> MAMITGGELVVRTLIKAGVEHLFGLHGAHIDTIFQACLDHDVPIIDTRHEAAAGHAAEGYARAGAKLGVALVTAGGGFTNAVTPIANAWLDRTPVLFLTGSGALRDDETNTLQAGIDQVAMAAPITKWAHRVMATEHIPRLVMQAIRAALSAPRGPVLLDLPWDILMNQIDEDSVIIPDLVLSAHGARPDPADLDQALALLRKAERPVIVLGSEASRTARKTALSAFVAATGVPVFADYEGLSMLSGLPDAMRGGLVQNLYSFAKADAAPDLVLMLGARFGLNTGHGSGQLIPHSAQVIQVDPDACELGRLQGIALGIVADVGGTIEALAQATAQDAAWPDRGDWCAKVTDLAQERYASIAAKSSSEHALHPFHASQVIAKHVDAGVTVVAD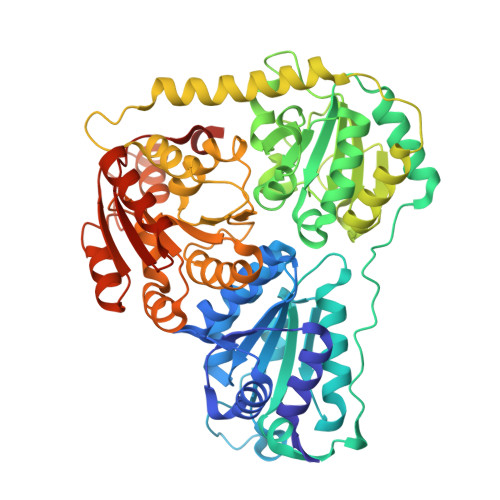GALTYLWLSEVMSRVKPGGFLCHGYLGSMGVGFGTALGAQVADLEAGRRTILVTGDGSVGYSIGEFDTLVRKQLPLIVIIMNNQSWGATLHFQQLAVGPNRVTGTRLENGSYHGVAAAFGADGYHVDSVESFSAALAQALAHNRPACINVAVALDPIPPEELILIGMDPFA Using genome-wide transcriptional and functional analyses combined with structural and population genetics studies, we conclusively demonstrated that a single amino acid change in the binding pocket of the glutathione-s-transferase epsilon 2 (GSTe2) gene, coupled with increased transcription, confers a high level of DDT resistance and also cross-resistance to pyrethroids in the major African malaria vector An. funestus. The topology of GSTe2 indicates that the 221 amino acids of the An. funestus GSTe2 (afGSTe2) are divided into two distinct domains similar to that of An. gambiae (92% similarity between the two species, with a difference of 20 amino acids). The active site is located in a deep cleft formed at the interface of the two domains, specifically by the interaction of H1 and H3 from the N-terminal domain and H4, H6 and H8 from the C-terminal domain. The active site of GSTe2 can be divided into two sub-sites.

To identify the structural changes responsible for the higher activity in the resistant GSTe2 Benin allele (119 F), its X-ray three-dimensional structure was determined and analyzed in comparison with that of a L119-GSTe2 susceptible allele cloned from Uganda (UG-GSTe2). Overall, the structure of BN-GSTe2 and UG-GSTe2 are very similar. However, significant local differences can be observed between the alleles at the C-terminal ends of H4 (containing the L119F mutation; residues from 113 to 128) and H8 (residues from 213 to 220). These differences can be described as a concerted movement of the BN-GSTe2 H4 and H8 helices with respect to those of UG-GSTe2, which opens the active site cleft. Leu119 normally forms part of the solvent-inaccessible hydrophobic core that stabilizes the conformation of helices H4, H5 and H8 of Uganda-GSTe2. However, to accommodate the bulkier Phe119 side chain in the Benin-GSTe2 structure, the N-terminal end of H4 has a dramatic bend, which increases the size of the H-site in comparison to the UG allele, where the cavity is tighter. The H-site surface representation of both proteins with a bound GSH confirms that the resistant BN allele has a larger putative DDT cavity than the susceptible UG allele. An assessment of the DDT dehydrochlorinase activity of the recombinant 119 F resistant enzyme (Benin) and that of susceptible L119 revealed that the 119 F allele is 3.4 times more efficient at metabolizing DDT (82.9% DDT depletion after 1 hr reaction in the presence of the cofactor glutathione (GSH); P < 0.001) than the L119 allele (24.4% depletion). This is confirmed by their respective kinetic parameters, with the 119 F allele having a higher catalytic efficiency (kcat/Km ratio) for DDT (316.3 μM−1.s−1 vs 92.0 μM−1.s−1). Overall, these structural analyses demonstrate that the L119F mutation is the causative mutation that confers DDT resistance.

>[2x]SHMTKLVLYTLHLSPPCRAVELTAKALGLELEQKNINLLAGDHLTPEFMKLNPQHTIPVLDDDGTIITESHAIMIYLVTKYGKDDTLYPKDPVQQARVNAALHFESGVLFARMRFIFERILFYGKSDIPEDRIEYVQKSYRLLEDTLKDDFVAGSKMTIADFSCISTISSIMGVVPLEQSEHPRIYEWIDRLKQLPYYEEANGGGGTDLGKFVLAKKEENAKA>MAKGTKYVSKVPDEHGFIEWSTEENLIWQELFTRQIACIKDKACDEYHEGLAKLNLPTDRIPQLDEVSKVLKVSTGWECYPVPALIGFGEFFRLLSEKKFPVATFIRSREEMDYLQEPDIFHEIFGHCPLLTNSSFANYTEAYGKMGLNATKEQRVFLARLYWFTIEFGLLDTPKGLRIYGGGVLSSPGETDYAMNNTDVDRKPFDILDVLRTPYRIDIMQPIYYMLTKVSDLDE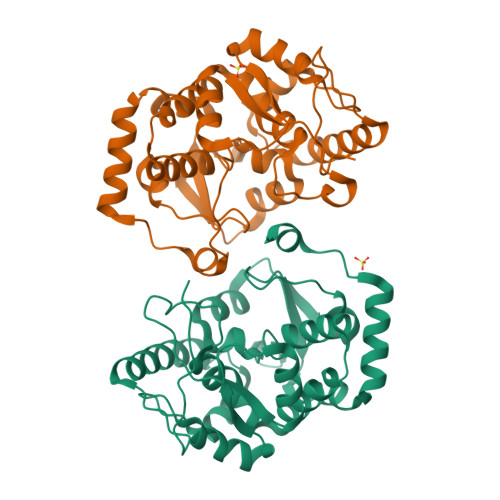IRKFEVDDIMELVAQAEALGLHEAKFPVKKASLEHHHHHH[2x]> MIRTWIALVPNDHRARLIGFALLAFCSVVARAVGTVLLVPLMAALFGEAPQRAWLWLGWLSAATVAGWVLDAVTARIGIELGFAVLNHTQHDVADRLPVVRLDWFTAENTATARQAIAATGPELVGLVVNLVTPLTSAILLPAVIALALLPISWQLGVAALAGVPLLLGALWASAAFARRADTAADKANTALTERIIEFARTQQALRAARRVEPARSLVGNALASQHTATMRLLGMQIPGQLLFSIASQLALIVLAGTTAALTITGTLTVPEAIALIVVMVRYLEPFTAVSELAPALESTRATLGRIGSVLTAPVMVAGSGTWRDGAVVPRIEFDDVAFGYDGGSGPVLDGVSFCLQPGTTTAIVGPSGCGKSTILALIA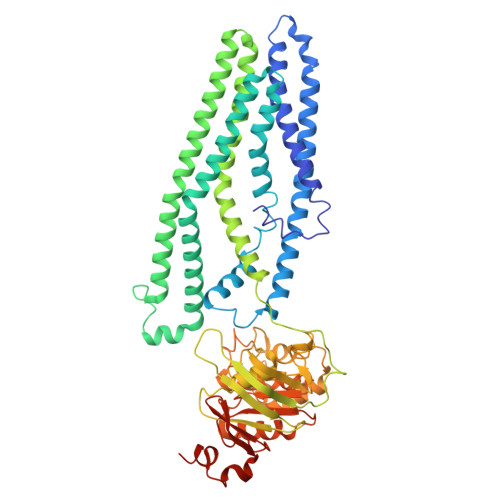GLHQPTRGRVLIDGTDVATLDARAQQAVCSVVFQHPYLFHGTIRDNVFAADPGASDDQFAQAVRLARVDELIARLPDGANTIVGEAGSALSGGERQRVSIARALLKAAPVLLVDQATSALDAENEAAVVDALAADPRSRTRVIVAHRLASIRHADRVLFVDDGRVVEDGSISELLTAGGRFSQFWRQQHEAAEWQILAE The Bacillus subtilis efflux pump BmrA, belongs to the type-IV family of MDR ABC transporters, conferring resistance to cervimycin-C secreted by the biotope competitor Streptomyces tendæ13. Type IV ABC transporters involved in MultiDrug Resistance (MDR) phenotype perform their function by undergoing a series of conformational changes pertaining to the alternating access mechanism. They are formed of two transmembrane domains (TMD) forming a cavity at their center where substrates bind, and of two nucleotide-binding domains (NBD) binding and hydrolyzing ATP-Mg2+ to fuel the system. Binding of ATP-Mg2+ to the NBDs bring them together, translating this conformational change to the TMDs which then open towards the outside (Outward-Facing, OF) where substrates are released. Importantly, the E504A catalytic mutant that still binds ATP but cannot hydrolyze it20 was used in this study; this thus allowed to probe a unidirectional transition from IF to OF states, BmrA being blocked when reaching the OF conformation when complexed with ATP-Mg2+ 9,12,14.

Interestingly, all ligands induce a cooperative ATP-Mg2+ binding like R6G, with a similar K0.5 (56.0 µM ± 2.6 h = 2.0 ± 0.3 for Hœchst33342; 65.5 µM ± 3.6 h = 2.3 ± 0.3 for Doxorubicin), suggesting a similar influence of ligands on ATP-Mg2+ binding, albeit the varying hill slope between ligands suggests that a ligand-specific effect might occur. We solved the cryoEM structure of E504 in complex with Hœchst33342 in absence of ATP-Mg2+ (named E504AH33342). Here again, E504AH33342 is 100% in the IF conformation. The high-resolution reconstruction differs slightly from E504Aapo, with a reorientation of the second half of the transporter induced by Hœchst-binding, leading to a further separation of the trans-membrane helices and a re-orientation of the second NBD. These modifications match the ones induced by R6G binding, with E504AH33342 structure being very similar to E504AR6G-25µMATP. Two molecules of Hœchst33342 bind per BmrA dimer, in a similar location as the one occupied by R6G. Ligand-binding on BmrA was similar within the drug-binding pocket, but extruding more within the TM helices for Hœchst33342, its structure being longer than R6G. Rotation of the NBD centered on V363 is reduced by half with only 6° sampled; rotation centered on E453 is impacted in a similar range as R6G with 4° sampled; finally, closure of the NBDs towards each other is abolished by Hœchst33342 binding, with 1 Å fluctuations observed corresponding to natural protein vibrations. Hœchst33342 also induces a reduction in the conformational space exploration of the NBDs, confirming the observations made on R6G, and showing a further decrease in amplitude compared to R6G.

>[2x]MSSSHHHHHHMPTKKQKSKSKLKPFFALVRRTNPSYGKLAFALALSVVTTLVSLLIPLLTKQLVDGFSMSNLSGTQIGLIALVFFVQAGLSAYATYALNYNGQKIISGLRELLWKKLIKLPVSYFDTNASGETVSRVTNDTMVVKELITTHISGFITGIISVIGSLTILFIMNWKLTLLVLVVVPLAALILVPIGRKMFSISRETQDETARFTGLLNQILPEIRLVKASNAEDVEYGRGKMGISSLFKLGVREAKVQSLVGPLISLVLMAALVAVIGYGGMQVSSGELTAGALVAFILYLFQIIMPMGQITTFFTQLQKSIGATERMIEILAEEEEDTVTGKQIENAHLPIQLDRVSFGYKPDQLILKEVSAVIEAGKVTAIVGPSGGGKTTLFKLLERFYSPTAGTIRLGDEPVDTYSLESWREHIGYVSQESPLMSGTIRENICYGLERDVTDAEIEKAAEMAYALNFIKELPNQFDTEVGERGIMLSGGQRQRIAIARALLRNPSILMLDAATSSLDSQSEKSVQQALEVLMEGRTTIVIAHRLSTVVDADQLLFVEKGEITGRGTHHELMASHGLYRDFAEQQLKMNADLENKAG>MNKWLDLILKIHVHPFLWIIAALGLLTGHMKALLCLLLIVLIHQLGHAALAVFFSWRIKRVFLLPFGGTVEVEEHGNRPLKEEFAVIIAGPLQHIWLQFAAWMLAEVSVIHQHTFELFTFYNLSILFVNLLPIWPLDGGKLLFLLFSKQLPFQKAHRLNLKTSLCFCLLLGCWVLFVIPLQISAWVLFVFLAVSLFEEYRQRHYIHVRFLLERYYGKNRELEKLLPLTVKAEDKVYHVMAEFKRGCKHPIIIEKSGQKLSQLDENEVLHAYFADKRTNSSMEELLLPYKLDYKDDDDKDYKDDDDKLEHHHHHH[2x];>[2x]MVTGVFAALGFVVKELVFLVSYVKNNAFPQPLSSSEEKKYLELMAKGDEHARNMLIEHNLRLVAHIVKKFENTGEDAEDLISIGTIGLIKGIESYSAGKGTKLATYAARCIENEILMHLRALKKTKKGSHHHHHH

S2P intramembrane metalloproteases regulate diverse signaling pathways across all three domains of life. Here we determine the cryo-EM structure of the S2P family intramembrane metalloprotease SpoIVFB from Bacillus subtilis bound to its native substrate Pro-σK. The structure and accompanying biochemical data demonstrate that SpoIVFB positions Pro-σK at the enzyme active site through a β-sheet augmentation mechanism, and reveal key interactions between Pro-σK and the interdomain linker connecting SpoIVFB transmembrane and CBS domains. Finally, the zinc-metalloprotease activity of SpoIVFB results in cleavage of the N-terminal pro-sequence of Pro-σK within the interior of the lipid membrane, allowing the mature σK to diffuse from the outer forespore membrane into the mother cell cytoplasm, bind to RNA polymerase core subunits, and initiate transcription of genes involved in the final stages of B. subtilis spore maturation (step 3).

An E44Q mutation in the HEXXH motif of SpoIVFB completely abolishes the proteolytic activity of the enzyme. To further investigate the overall architecture of detergent-solubilized SpoIVFB and Pro-σK preparations, we pursued cryo-EM reconstructions of both WT and E44Q SpoIVFB co-purified with Pro-σK. Aside from the difference in oligomeric state, which we believe arises simply from variations between protein preparations and fragile monomer interfaces, the final structures of WT and E44Q SpoIVFB:Pro-σK monomers are virtually superimposable (RMSD ~ 0.5 Å). While the orientation of zinc-coordinating residues H43, H47, and D137 of SpoIVFB are conserved with those of mjS2P, the cryo-EM map of WT SpoIVFB:Pro-σK does not show any appreciable density for an ion being coordinated by these residues. This lack of density was consistent in the cryo-EM maps of both WT and E44Q SpoIVFB:Pro-σK, demonstrating that SpoIVFB:Pro-σK complexes fail to co-purify with the Zn2+ ion that is essential for supporting Pro-σK cleavage. In both our WT and E44Q SpoIVFB:Pro-σK preparations the purified protein is devoid of the catalytic zinc ion. In this work we identified dimeric, trimeric, and tetrameric oligomeric states of the SpoIVFB: Pro-σK complex. We believe that these oligomeric states are likely an artifact of detergent solubilization and weak lipid/detergent interactions between monomers in the purified protein preparations.>[2x]MAAPTPEEVRQMYDDFTDPFARIWGENLHFGYWEDAGADVSVDDATDRLTDEMIALLDVRSGDRVLDVGCGIGKPAVRLATARDVRVTGISISRPQVNQANAR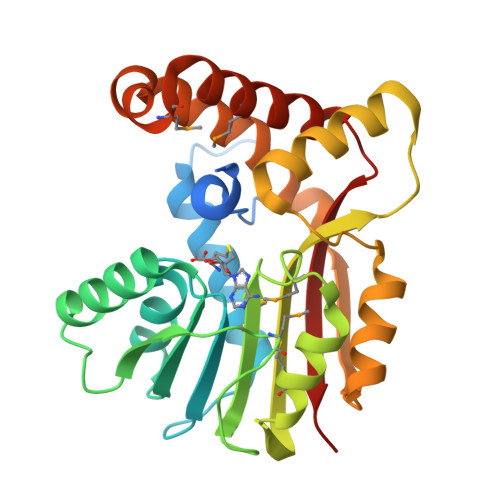ATAAGLANRVTFSYADAMDLPFEDASFDAVWALESLHHMPDRGRALREMARVLRPGGTVAIADFVLLAPVEGAKKEAVDAFRAGGGVLSLGGIDEYESDVRQAELVVTSTVDISAQARPSLVKTAEAFENARSQVEPFMGAEGLDRMIATFRGLAEVPEAGYVLIGARKP> WSADERQRMLVQRKDELLQQ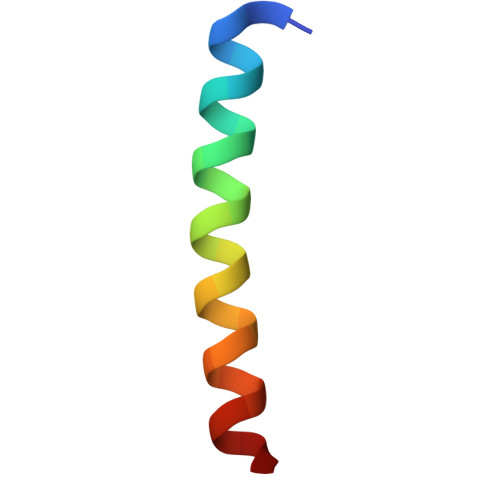ARKRFLNK>GHH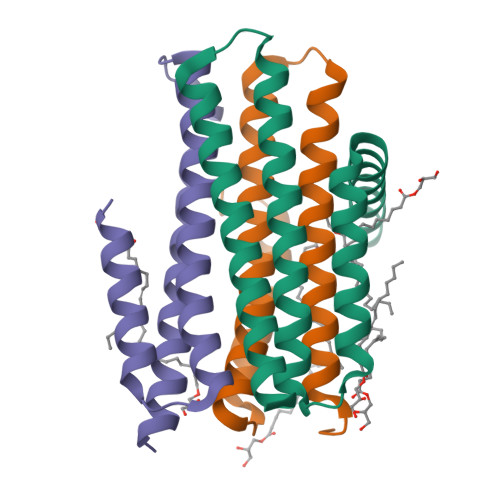HHHHELANNTTGFTRIIKAAGYSWKGLRAAWINEAAFRQEGVAVLLCVVIAAWLDVDAVTRVLLISSVMLVMIVELLNSAIEAVVDRIGSEYHELSGRAKDLGSAAVLIAIIDAVITWAILLWSHFG[6x]>RPGADCEVCKEFLNRFYKSLIDRGVNFSLDTIEKELISFCLDTKGKENRLCYYLGATKDAATKILSEVTRPMSVHMPAMKICEKLKKLDSQICELK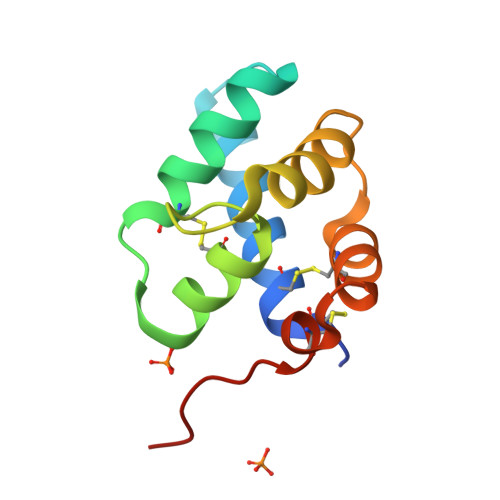YEKTLD[2x]>GMVKDKNDVGPKTVAILGAG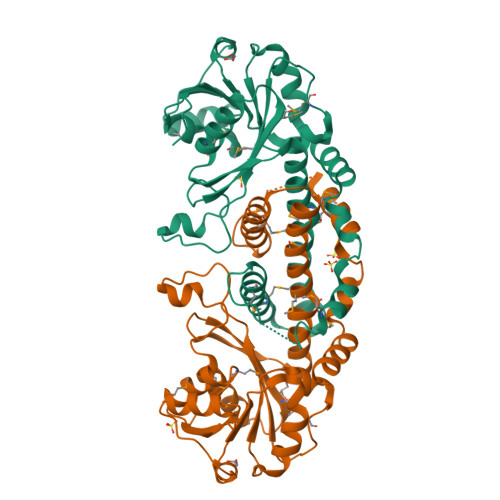GKMGARITRKIHDSAHHLAAIEIAPEGRDRLQGMGIPLTDGDGWIDEADVVVLALPDNIIEKVAEDIVPRVRPGTIVLILDAAAPYAGVMPERADITYFIGHPCHPPLFNDETDPAARTDYHGGIAKQAIVCALMQGPEEHYAIGADICETMWSPVTRTHRVTTEQLAILEPGLSEMVAMPFVETMVHAVDECADRYGIDRQAALDFMIGHLNVEIAMWFGYSPKVPSDAALRLMEFAKDIVVKEDWREALNPAKVKQAAELIAGK[2x]> MATLLRSLALFKRNKDKPPITSGSGGAIRGIKHIIIVPIPGDSSITTRSRLLDRLVRLIGNPDVSGPKLTGALIGILSLFVESPGQLIQRITDDPDVSIRLLEVVQSDQSQSGLTFASRGTNMEDEADQYFSHDDPISSDQSRFGWFENK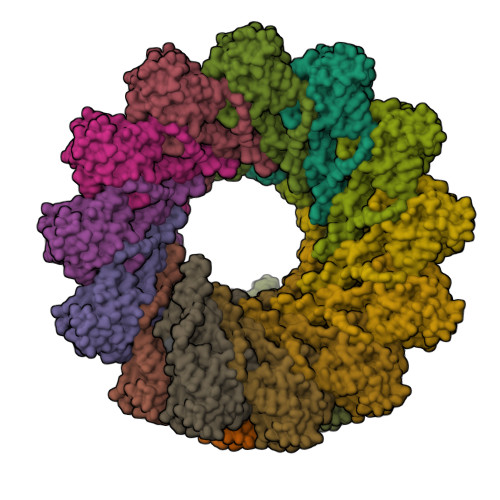EISDIEVQDPEGFNMILGTILAQIWVLLAKAVTAPDTAADSELRRWIKYTQQRRVVGEFRLERKWLDVVRNRIAEDLSLRRFMVALILDIKRTPGNKPRIAEMICDIDTYIVEAGLASFILTIKFGIETMYPALGLHEFAGELSTLESLMNLYQQMGETAPYMVILENSIQNKFSAGSYPLLWSYAMGVGVELENSMGGLNFGRSYFDPAYFRLGQEMVRRSAGKVSSTLASELGITAEDARLVSEIAMHTTEDKVEHHHHHHHH We apply this method to identify inhibitors of ROCK1 from almost one billion commercially available compounds. To facilitate further validation of the method and confirm the postulated binding modes, we obtained co-crystal structures of ROCK1 in complex with Compound 1, the most potent inhibitor identified in the virtual screening campaign, and with Compound 22, an inhibitor we considered structurally unique. The crystals contained four monomers of the ROCK1 kinase domain in the asymmetric unit, of which chains A, B, and C were relatively well defined, while the fourth copy of chain D was quite poorly ordered and not used in analyses. Focusing on the chain A example in each structure, the resulting electron density shows a clear binding mode for each ligand.

The second structurally characterized inhibitor, Compound 22, and its analogs, contain a tetrahydropyridine linking group, which were not found in our survey of PDB kinase inhibitor structures. The three azaindole inhibitors have a distinctive tetrahydropyridine ring linking the putative hinge-binding group with the atoms that interact with the P-loop. The structures were solved and refined to a final resolution of 2.34 Å (Compound 1) and 2.74 Å (Compound 22). Analogously for Compound 22, the azaindole nitrogen atoms involved in hydrogen bond interactions to the kinase hinge are only 0.4 or 1.0 Å displaced between the experimental and docked poses. In this case, the displacement between the two molecules becomes larger as one moves distally to the hinge towards the back portion of the pocket underneath the P loop. For example, the carbonyl group on the docked ligand that interacts with the tip of the conserved kinase N lobe lysine 105 is displaced 1.8 Å from the experimental structure and the respective distal phenyl groups underneath the P loop are 3.4 Å apart. However, it is critical to note that the protein itself demonstrates shifts of similar size in our alignment, such that we observe displacements between our experimental structure and that used as a template in the docking procedure of 2.1 Å at the zeta nitrogen of Lys105 and 2.4 Å for equivalent backbone C-alphas (Phe87) at the P loop turn, or a 4.2 Å difference at the outer tip of that phenylalanine 87 sidechain. These observations suggest that the bulk of the observed ligand displacement is due to the malleability and differences in the protein component that the docking algorithms would not be expected to achieve. For instance, ROCK1’s helix C is partially unwound in the mid-section affording greater plasticity and this directly abuts the P loop and outer portions of the binding pocket. It is again reassuring that given those large adjustments in the protein, the ligand binding conformation itself is quite well matched between the two models, albeit with this tilted trajectory differential.

>ASFETRFEKMDNLLRDPKSEVNSDCLLDGLDALVYDLDFPALRKNKNIDNFLSRYKDTINKIRDLRMKAEDYEVVKVIGRGAFGEVQLVRHKSTRKVYAMKLLSKFEMIKRSDSAFFWEERDIMAFANSPWVVQLFYAFQDDRYLYMVMEYMPGGDLVNLMSNYDVPEKWARFYTAEVVLALDAIHSMGFIHRDVKPDNMLLDKSGHLKLADFGTCMKMNKEGMVRCDTAVGTPDYISPEVLKSQGGDGYYGRECDWWSVGVFLYEMLVGDTPFYADSLVGTYSKIMNHKNSLTFPDDNDISKEAKNLICAFLTDREVRLGRNGVEEIKRHLFFKNDQWAWETLRDTVAPVVPDLSSDIDTSNFDDLEEDKGEEETFPIPKAFVGNQLPFVGFTYYSN[4x]> TMLCVLTTDAAAEPAALERALRRAAAATFDRLDIDGSCSTNDTVLLLSSGASEIPPAQADLDEAVLRVCDDLCA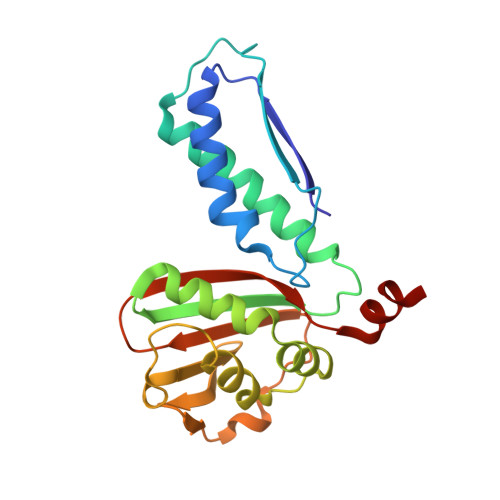QLQADAEGVTKRVTVTVTGAATEDDALVAARQIARDSLVKTALFGSDPNWGRVLAAVGMAPITLDPDRISVSFNGAAVCVHGVGAPGAREVDLSDADIDITVDLGVGDGQARIRTTDLSHAYVEENSAYSS> MSLKDKKILIVEDSKFQAKTIANILNKYGYTVEIALTGEAAVEKVSGGWYPDLILMDIELGEGMDGVQTALAIQQISELPVVFLTAHTEPAVVEKIRSVTAYGYVMKSATEQVLITIVEMALRLYEANVHANE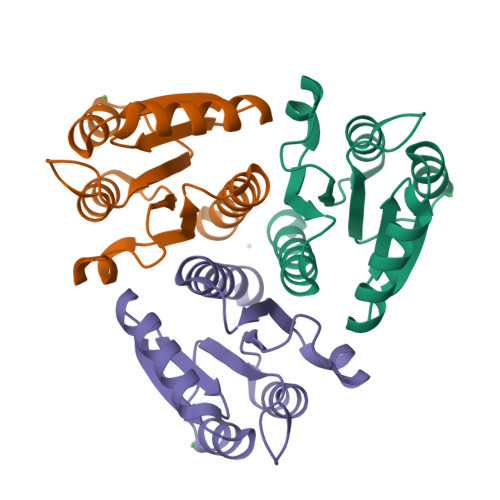GHHHHHH>GSHMDASVMSTTYALSAAQTEIWLAQQLYPDSPVYNIAQYTVIEGVIEPAVFEAALRQVIDEADTLRLQFIDSDDGLRQRIGTPAWSMPVLDLTAQADPQAAAQAWMRADYQQPVNLTQGPLFCYALLKVAPAQWMWYQRYHVIMMDGYGAYLIAQRVAYVYSALCEGTTPAECDFGSILQLLESDAQYQISAQRAQDEAYWLKHCANWSEPATLASRSAPVLQQRLRQTTYLAIQALGDTAPDARRLAQFMTAAMAAYLYRFTGEQDVVLGLPVK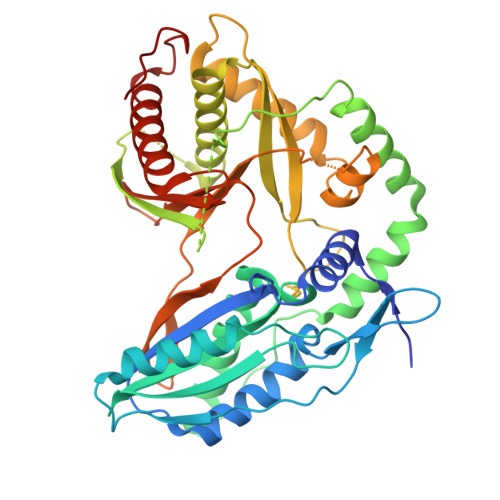VRFGADRHIPGMKSNTLPLRLTMRPGMNLSSLMQQAAQEMQSGLRHQRYPSEALRRQLGMPSGQRLFGTTVNVMPFDLDLSFGGYSATNHNLLNGPAEDLMLGVYWTPGSHQLRIDFDANPACYTPEGLGAHQRRFIRFMQVLAADATQPIDSIDLLD[4x]>MTMVGLIWAQATSGVIGRGGDIPWRLPEDQAHFREITMGHTIVMGRRTWDSLPAKVRPLPGRRNVVLSRQADFMASGAEVVGSLEEALTSPETWVIGGGQVYALALPYATRCEVTEVDIGLPREAGDALAPVLDETWRGETGEWRFSRSGLR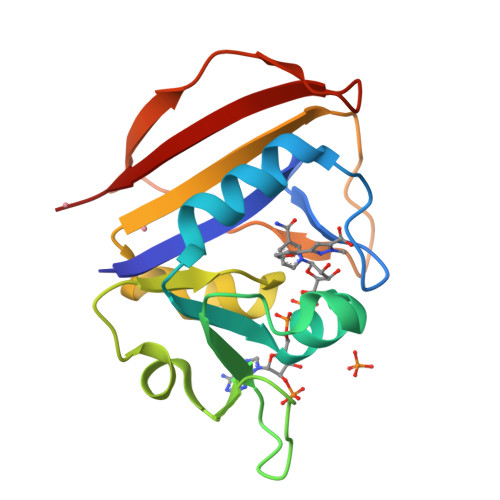YRLYSYHRS[2x]(S)-1-(4-methoxyphenyl)-1-(1-methyl-1H-imidazol-2-yl)methanamine | C12 H15 N3 O 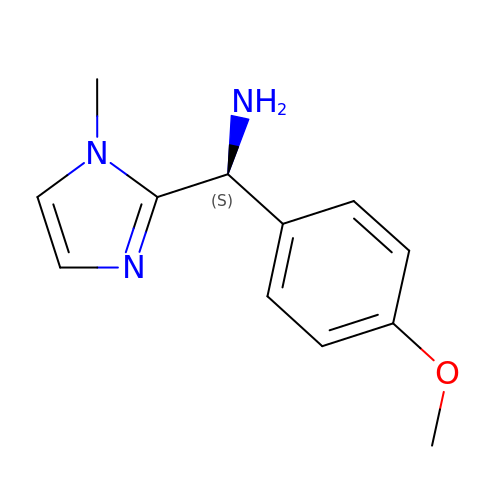| NGFVORJRIAJDAY-NSHDSACASA-N> GPGSELPQMVQQLNSPDQQELQSALWKLRNIASGGNEQIQAVIDAGALPALVQLLSSPNEQILSSALGALSNIASGGNEQIQAVIDAGALPALVQLLSSPNEQILQLALWALSNIASGGNEQIQAVIDAGALPALVQLLSSPNEQILQEALWALSNIASGGNEQIQAVIDAGALPALVQLLSSPNEQILQEALWALSNIASGGNEQIQAVIDAGALPALVQLLSSPNEQILQEALWALSNIASGGNEQKQAVKEAGALEKLEQL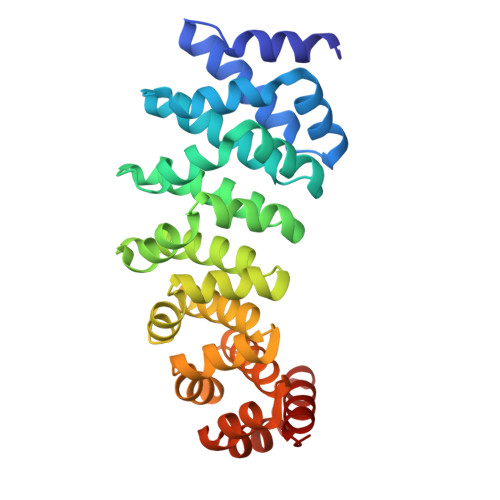QSHENEKIQKEAQEALEKLQSH(R)-N-(3-(1H-indol-3-yl)-1-oxo-1-(pyridin-4-ylamino)propan-2-yl)-4-(4-(3,4-difluorophenyl)piperazin-1-yl)-2-fluorobenzamide 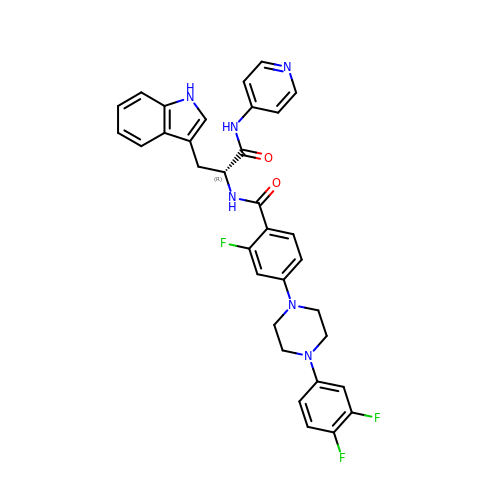| C33 H29 F3 N6 O2 | UJJHTUJDTNONGY-WJOKGBTCSA-N>GNWLSTKALEQQTRDIPIEPKRGTIYDRNMKELAVSVTKYTVWCKPVEVEDKKEAAEKVAEILDEDYKDIYALISKKNMALVKVKRWIDDDKASQIRDAKLSGIWVAEDNQRYYPYGNFAPYVLGHTSSDATGISGVEMQYDKKLKGKPGKLIVSTDASGREIPQGMEKYYEPVQGNGLVLSIDEVIQHYTEKAVQKAYELNNAKKVTAIAMNPKTGDILALASKPDYDPNDSRTPIYPYYQEELEKYNDKDKIKGYYQMWRNPAVSDTYEPGSTFKLITSSSALEEGVIKDGEKFTCTGSVTVGGRKIKCWRHYRPHGTQEFKQAVQNSCNPVFVELGSRLGVGKMYDYIESFGLM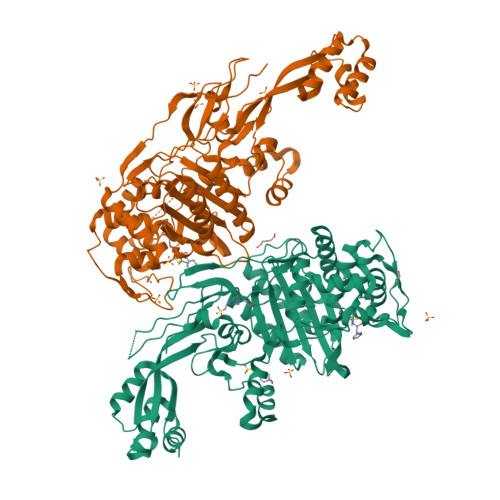DKTGIDLPGEAKGILYNEKNVGPVELATISFGQSISVTPIQLITAISSIANGGDLMQPRVVKSYTDNKGNITETVKPKKVRSVISKETSKKMLEIAESVVTEGGGKIAYIPGYRLGGKTGTAQKVIDGKYAPGKYICSFVGIAPCDDPQIVVLAIVDEPTGVSAFGSTTAGPIVKEIMNDSLKYLGVKPVY[2x]Uniquely, the sulfonylurea receptors SUR1 and SUR2 lack transport activity per se but instead are devoted to forming the ATP-sensitive potassium (KATP) channels, wherein four SUR.x subunits form a complex with four subunits of an inwardly rectifying potassium channel, Kir6.1 or Kir6.2. KATP channels are gated by intracellular ATP and ADP, key features which enable them to regulate membrane excitability according to the energetic state of the cell. In pancreatic β-cells, KATP channels composed of SUR1 and Kir6.2 couple glucose metabolism to insulin secretion. The SUR1 protein has an N-terminal transmembrane domain referred to as TMD0 that interacts directly with the Kir6.2 subunit, followed by a cytoplasmic loop termed L0, and then the ABC core structure comprising two transmembrane domains TMD1 and TMD2 and two nucleotide binding domains NBD1 and NBD2.

Further, as an additional control we determined the structure of channels without any pharmacochaperone or ATP (referred to as the apo state). Interestingly, the dominant class emerging from 3D classification for the ATP-only state as well as the apo state presented a similar conformation, with Kir6.2 tetramer closed and SUR1 inward-facing. Of note, a dominant inward-facing conformation in the absence of ligand was also observed in another ABC transporter, the multidrug resistance protein MRP1. These observations suggest the closed channel conformation is the most stable for the apo state under our experimental conditions (i.e. no ATP and no exogenous PIP2, a lipid required for KATP channel opening [Nichols, 2006]). Here, in both the RPG/ATP and CBZ/ATP structures, we observe strong and distinctly shaped cryo-EM densities within the same GBC binding pocket. Such density is absent in the ATP-only and the apo structures, supporting assignment as the pharmacochaperone ligand. By contrast, the KNt cryoEM density is absent in the apo structure, suggesting that when no ATP is bound to Kir6.2, KNt has little residence time in the ABC core central cavity. The fact that despite not seeing KNt, the Kir6.2 channel is still closed in the dominant class structure is likely due to loss of endogenous PIP2 during purification.

> MPLAFCGTENHSAAYRVDQGVLNNGCFVDALNVVPHVFLLFITFPILFIGWGSQSSKVHIHHSTWLHFPGHNLRWILTFILLFVLVCEIAEGILSDGVTESRHLHLYMPAGMAFMAAITSVVYYHNIETSNFPKLLIALLIYWTLAFITKTIKFVKFYDHAIGFSQLRFCLTGLLVILYGMLLLVEVNVIRVRRYIFFKTPREVKPPEDLQDLGVRFLQPFVNLLSKGTYWWMNAFIKTAHKKPIDLRAIAKLPIAMRALTNYQRLCVAFDAQARKDTQSPQGARAIWRALCHAFGRRLILSSTFRILADLLGFAGPLCIFGIVDHLGKENHVFQPKTQFLGVYFVSSQEFLGNAYVLAVLLFLALLLQRTFLQASYYVAIETGINLRGAIQTKIYNKIMHMSTSNLSMGEMTAGQICNLVAIDTNQLMWFFFLCPNLWTMPVQIIVGVILLYYILGVSALIGAAVIILLAPVQYFVATKLSQAQRTTLEHSNERLKQTNEMLRGMKLLKLYAWESIFCSRVEVTRRKEMTSLRAFAVYTSISIFMNTAIPIAAVLITFVGHVSFFKESDLSPSVAFASLSLFHILVTPLFLLSSVVRSTVKALVSVQKLSEFLSSAEIREEQCAPREPAPQGQAGKYQAVPLKVVNRKRPAREEVRDLLGPLQRLAPSMDGDADNFCVQIIGGFFTWTPDGIPTLSNITIRIPRGQLTMIVGQVGCGKSSLLLATLGEMQKVSGAVFWNSNLPDSEGEDPSSPERETAAGSDIRSRGPVAYASQKPWLLNATVEENITFESPFNKQRYKMVIEACSLQPDIDILPHGDQTQIGERGINLSGGQRQRISVARALYQQTNVVFLDDPFSALDVHLSDHLMQAGILELLRDDKRTVVLVTHKLQYLPHADWIIAMKDGTIQREGTLKDFQRSECQLFEHWKTLMNRQDQELEKETVMERKASEPSQGLPRAMSSRDGLLLDEEEEEEEAAESEEDDNLSSVLHQRAKIPWRACTKYLSSAGILLLSLLVFSQLLKHMVLVAIDYWLAKWTDSALVLSPAARNCSLSQECDLDQSVYAMVFTLLCSLGIVLCLVTSVTVEWTGLKVAKRLHRSLLNRIILAPMRFFETTPLGSILNRFSSDCNTIDQHIPSTLECLSRSTLLCVSALTVISYVTPVFLVALLPLAVVCYFIQKYFRVASRDLQQLDDTTQLPLVSHFAETVEGLTTIRAFRYEARFQQKLLEYTDSNNIASLFLTAANRWLEVCMEYIGACVVLIAAATSISNSLHRELSAGLVGLGLTYALMVSNYLNWMVRNLADMEIQLGAVKRIHALLKTEAESYEGLLAPSLIPKNWPDQGKIQIQNLSVRYDSSLKPVLKHVNTLISPGQKIGICGRTGSGKSSFSLAFFRMVDMFEGRIIIDGIDIAKLPLHTLRSRLSIILQDPVLFSGTIRFNLDPEKKCSDSTLWEALEIAQLKLVVKALPGGLDAIITEGGENFSQGQRQLFCLARAFVRKTSIFIMDEATASIDMATENILQKVVMTAFADRTVVTIAHRVHTILSADLVMVLKRGAILEFDKPETLLSQKDSVFASFVRADK>VRSSSRTPSDKPVAHVVANPQAEGQLQWLNRRANALLANGVELRDNQLVVPSEGLYLIYSQVLFKGQGCPSTHVLLTHTISRIAVSYQTKVNLLSAIKSPCQRETPEGAEAKPWYEPIYLGGV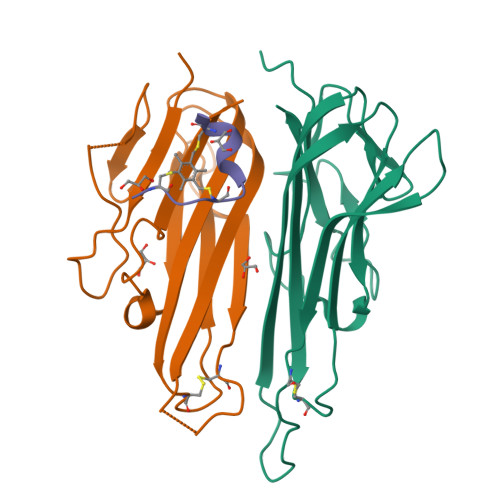FQLEKGDRLSAEINRPDYLDFAESGQVYFGIIAL[4x];>ACPPCLWQVLCG[2x]~{N}-[[2,2-bis(fluoranyl)-10,12-dimethyl-1,3-diaza-2$l^{4}-boratricyclo[7.3.0.0^{3,7}]dodeca-4,6,9,11-tetraen-4-yl]methyl]ethanamide | C14 H17 B 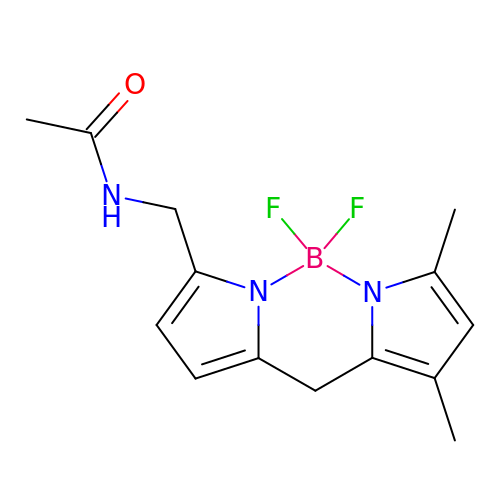F2 N3 O | ICEVSDSYCIWMTJ-UHFFFAOYSA-N> MNRRDFLKGIASSSFVVLGGSSVLTPLNALAKAGINEDEWLTTGSHFGAFKMKRKNGVIAEVKPFDLDKYPTDMINGIRGMVYNPSRVRYPMVRLDFLLKGHKSNTHQRGDFRFVRVTWDKALTLFKHSLDEVQTQYGPSGLHAGQTGWRATGQLHSSTSHMQRAVGMHGNYVKKIGDYSTGAGQTILPYVLGSTEVYAQGTSWPLILEHSDTIVLWSNDPYKNLQVGWNAETHESFAYLAQLKEKVKQGKIRVISIDPVVTKTQAYLGCEQLYVNPQTDVTLMLAIAHEMISKKLYDDKFIQGYSLGFEEFVPYVMGTKDGVAKTPEWAAPICGVEAHVIRDLAKTLVKGRTQFMMGWCIQRQQHGEQPYWMAAVLATMIGQIGLPGGGISYGHHYSSIGVPSSGAAAPGAFPRNLDENQKPLFDSSDFKGASSTIPVARWIDAILEPGK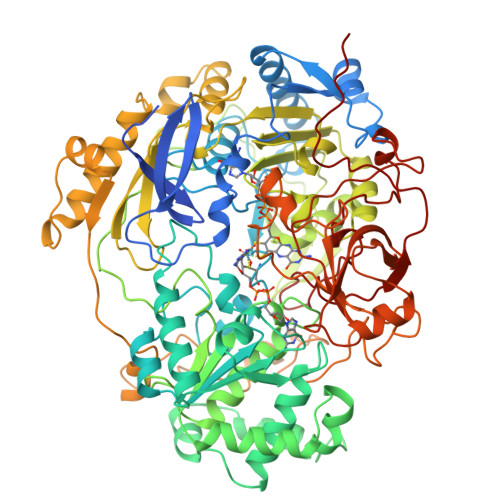TIDANGSKVVYPDIKMMIFSGNNPWNHHQDRNRMKQAFHKLECVVTVDVNWTATCRFSDIVLPACTTYERNDIDVYGAYANRGILAMQKMVEPLFDSLSDFEIFTRFAAVLGKEKEYTRNMGEMEWLETLYNECKAANAGKFEMPDFATFWKQGYVHFGDGEVWTRHADFRNDPEINPLGTPSGLIEIFSRKIDQFGYDDCKGHPTWMEKTERSHGGPGSDKHPIWLQSCHPDKRLHSQMCESREYRETYAVNGREPVYISPVDAKARGIKDGDIVRVFNDRGQLLAGAVVSDNFPKGIVRIHEGAWYGPVGKDGSTEGGAEVGALCSYGDPNTLTLDIGTSKLAQACSAYTCLVEFEKYQGKVPKVSSFDGPIEVEI>GSHMARIASALDNVSANVMIADNDLNIIYMNRTVSEMLGRAEADIRKQLPNFDAGRLMGANIDVFHKNPAHQRHLLANLTGVHKAELNLGGRRFSLDVVPVFNDAN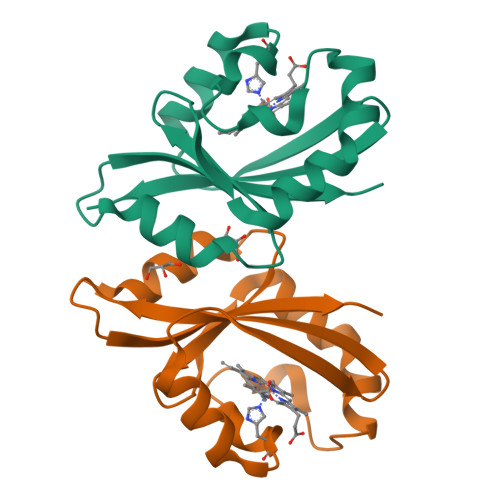ARLGSAVQWTDRTEE[4x]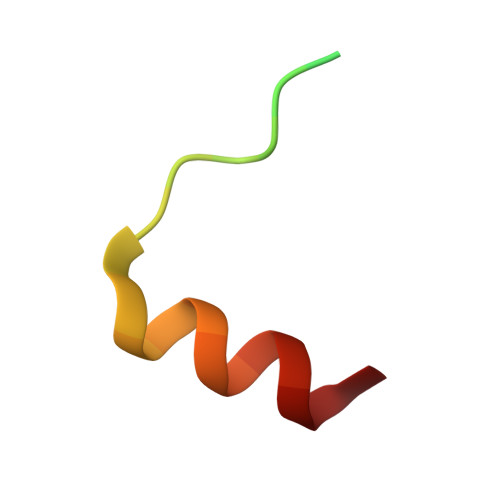> KEKARAMRVNKRAPQMDWNRKREIFSNF6,6'-heptane-1,7-diylbis(4-methylpyridin-2-amine) | C19 H28 N4 | 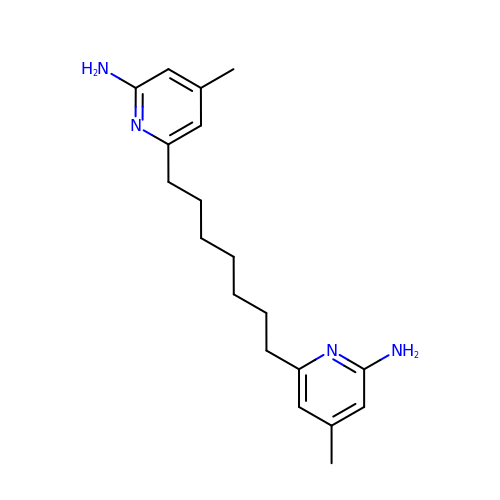FSVLONGGRYPEKX-UHFFFAOYSA-N> SNAQIAAVDPAGMSVIRDRNQLFRVNSAGEVENTYTLKVINKTQQVQEYNLDVKGLNDVSWYGKQTIQVEPGEVLNLPMSLGADPDKLNSAITTIQFILTDKSN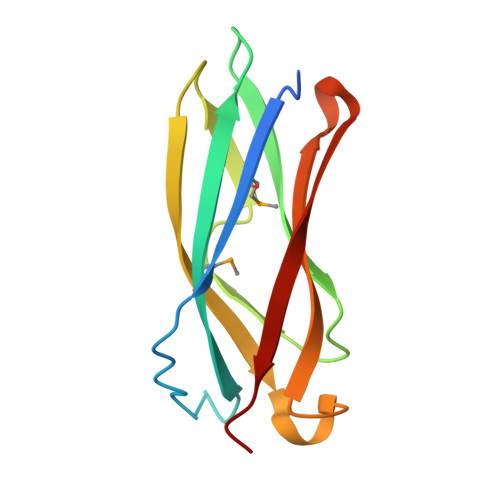EFTIEVESRFIKKL> SNAGFQQSHYFVALYRFKALEK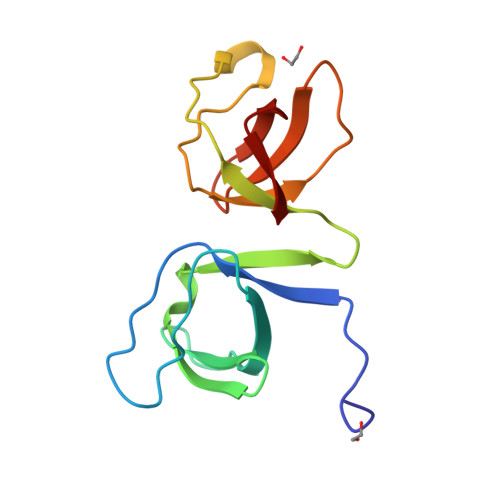DDLDFRPGEKITVIDDSNEESWRGKIGEKVGFFPPNFIIRVRAGERVHRVTRSFVGNREIGQITLKKDQIVVQKGDEAGGYVKVYTGRKVGLFPTDFLEEI>[2x]MSFMDQIPGGGNYPKLPVECLPNFPIQPSLTFRGRNDSHKLKNFISEIMLNMSMISWPNDASRIVYCRRHLLNPAAQWANDFVQEQGILEITFDTFIQGLYQHFYKPPDINKIFNAITQLSEAKLGIERLNQRFRKIWDRMPPDFMTEKAAIMTYTRLLTKETYNIVRMHKPETLKDAMEEAYQTTALTERFFPGFELDADGDTIIGATTHLQEEYDSDYDSEDNLTQNRYVHTVRTRRSYNKPMSNHRNRRNNNASREECIKNRLCFYCKKEGHRLNECRARKAVLTDLELESKDQQTLFIKTLPIVH

Here, we have determined the structure and molecular architecture of the Ty3 capsid by 3D and 2D cryo-electron microscopy (cryo-EM) and compared it with those of the retroviruses. In the case of Ty3, Gag3 is cleaved into CA and NC domains. Formation of the capsid is important for genome protection and is an essential step in the retroelement life cycle. Similar to retroviruses, the protruding capsomers of the Ty3 capsid are formed by the CA-NTD, while the inner layer, linking the capsomers together, is formed by the CA-CTD.

The densities for the nine non–symmetry-related copies of the Ty3 CA-CTD were aligned and averaged to generate a higher resolution 4.9-Å map. The homology model of the Ty3 CA-CTD was then flexibly fitted into the map and showed very good agreement with the density. We observed protrusions from the EM densities around the α-helices, at positions corresponding to the large side chains (F134, R135, W138, R157, and Y164), confirming the quality of the model and the fit. We were also able to trace the very C-terminal short part of the CA-CTD, which appears to interact with the neighboring CA-CTD. The mutations (E190A/R191A) in that region cause a strong phenotype in yeast. These mutant Ty3 particles form long filaments in cells, instead of spherical particles, indicating that the C-terminal part of Ty3 CA-CTD is important for the capsid assembly. CA CTD–CTD interactions at the dimeric and trimeric interfaces showed a continuum of differing relative orientations. Strikingly, the quaternary arrangement of the PR- Ty3 CA-CTDs is almost identical to that of the CA-CTD in mature HIV-1 capsids at the level of dimer, trimer, and even pentamer. Despite the similarity in the CA-CTD quaternary packing, there is very little conservation of residues at protein–protein interfaces.> LRPLR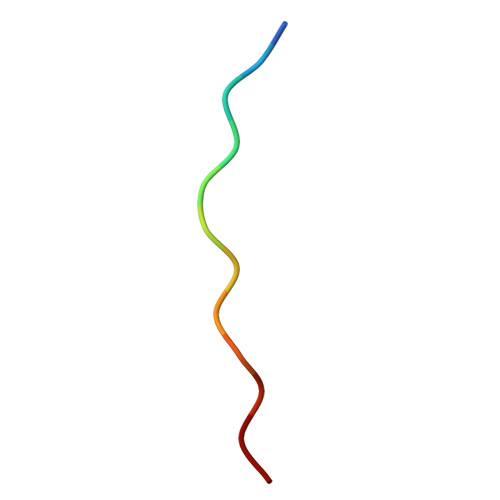PLRPLRP>[12x]XXXXXXXXXXXXXXXXXXXXXXXXXXXXXXXXXXXXILIATKDDLTKQ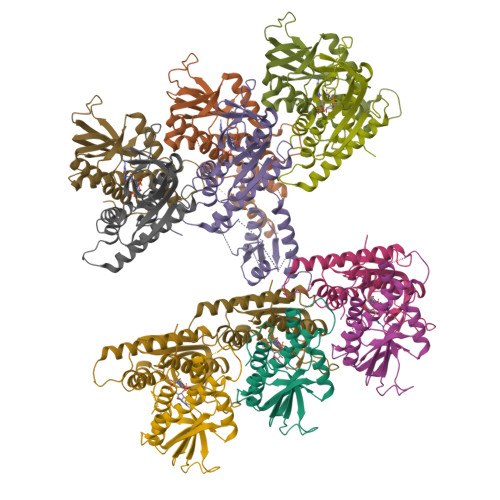RGESLTKPRDNVVFEFGLFLGAAGPEKCYLIAEXXXXXXXXXXXXXXXXXXXEDTDLPTDLDGITVAKFTRNSGQYNSLDKIVESIRTHLVKIAEMSQLGLLPSTALAIGYYNSFIKRVCEEIHGSECVELEGKKIKVKSFRVDVVIPETLDDNGVGNFTTLYNKRYGLSKATTCTNPALLGTRGFPFHFKVDPPDANQESPVDIHLLDIPSTLSTIVESLKLYLPSNQVGQDFDMDYLEMRELENFAKVLKYLIGRNAATKGYVNVLTNVKL> GSHMTIEQMVDRLLSYPERTKMQILAPIVSGKKGTHAKTLEDIRKQGYVRVRIDREMRELTGDIELEKNKKHSIDVVVDRIIIKDGIAARLADSLETALKLADGKVVVDVIGEGELLFS;> GSHMGSPEEYRELVVSLRVGMEIERNALLRRLVDIQYDRNDIDFRRGTFRVRGDVVEIFPASRDEHCIRVEFFGDEIERIREVDALTGEVLGEREHVAIFPAS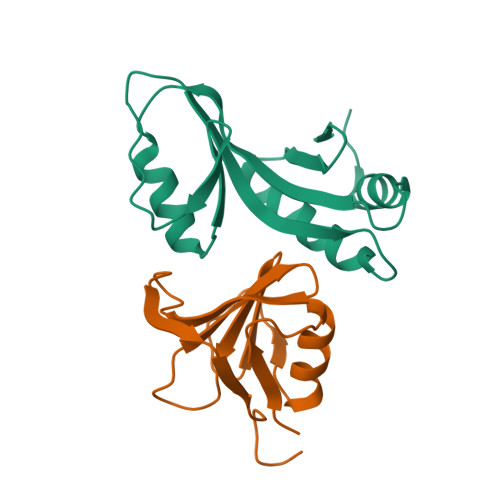HFV>[2x]SNAMKELIKEHQKDINPALQLHDWVEYYRPFAANGQSANYIPALGKVNDSQLGICVLEPDGTMIHAGDWNVSFTMQSISKVISFIAACMSRGIPYVLDRVDVEPTGDAFNSIIRLEINKPGK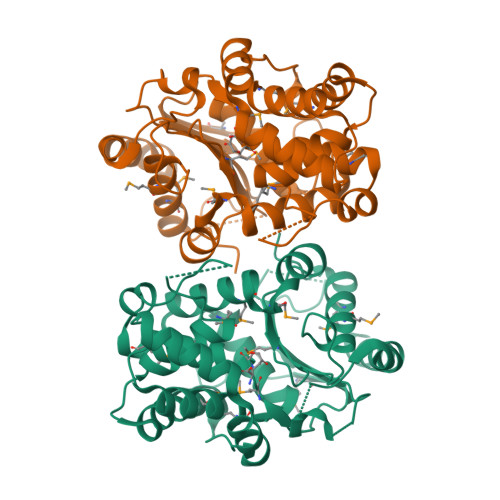PFNPMINAGALTIASILPGESAYEKLEFLYSVMETLIGKRPRIHEEVFRSEWETAHRNRALAYYLKETNFLEAEVEETLEVYLKQCAMESTTEDIALIGLILAHDGYHPIRHEQVIPKDVAKLAKALMLTCGMYNASGKYAAFVGVPAKSGVSGGIMALVPPSARREQPFQSGCGIGIYGPAIDEYGNSLTGGMLLKHMAQEWELSIF>[4x]TIFEERHLKYISQLGKGNFGSVELCRYDPLGDNTGALVAVKQLQHSGPDQQRDFQREIQILKALHSDFIVKYRGVSYGPGRQSLRLVMEYLPSGCLRDFLQRHRARLDASRLLLYSSQICKGMEYLGSRRCVHRDLAARNILVESEAHVKIADFGLAKLLPLDKDYYVV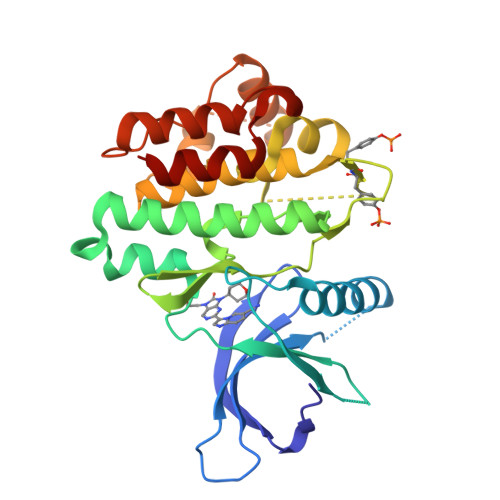REPGQSPIFWYAPESLSDNIFSRQSDVWSFGVVLYELFTYCDKSCSPSAEFLRMMGCERDVPALSRLLELLEEGQRLPAPPACPAEVHELMKLCWAPSPQDRPSFSALGPQLDMLW> YRVPKEVRVEPQKFAEE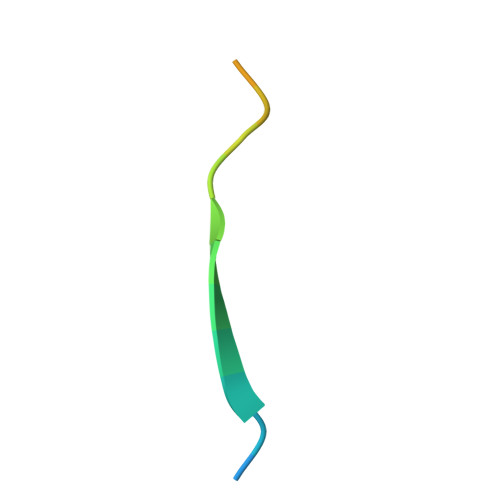LIH We have biochemically and structurally characterized a minimalist inositol phosphate kinase (i.e., TvIPK) encoded by Terrestrivirus, a nucleocytoplasmic large (“giant”) DNA virus (NCLDV). We show that TvIPK can synthesize inositol pyrophosphates from a range of scyllo- and myo-IPs, both in vitro and when expressed in yeast cells. We find a heart-shaped ligand binding pocket comprising an array of positively charged and flexible side chains, underlying the observed substrate diversity. A crucial arginine residue in a conserved “G-loop” orients the γ-phosphate of ATP to allow substrate pyrophosphorylation.

To gain an atomic level understanding of the ability of TvIPK to synthesize PP-IPs, we derived crystals of TvIPK17-265 in complex with ADP (1.95 Å resolution; Table EV1). For each asymmetric unit, there is one molecule of TvIPK17-265 in the C2221 space group. The N-terminal residues 17–47 could not be traced, either in this crystal complex, or in a binary complex of full-length TvIPK plus ADP, or in a number of TvIPK17-265/ADP complexes into which we soaked a variety of inositol phosphates (Table EV1, B and EV2A).

> DITNMSNIDLQSSKSVADEVIADIAEIVNKESIRIFPRIAGRSYIIYGQTSGIICKRMEKSDNEFVIYNYISEHYDKFLKKYVPKLYGKNNDMLLLEDLTYNYNNPNVMDVKIGARKRKSHTSGFFSIRGYTNSHDYKFDPDEYLTSESTINHIKNFMEAGGENRDKTKQVLLKWIMKLSELANDLFEINLKFDGVSLIFIYDDDCSKCDVNVVDFSRVKLIDTNDQMTISAVTNLIKILSELADNPLN Peptidyl-prolyl isomerases (PPIases) catalyze cis/trans isomerization of peptidyl-prolyl bonds, which is often rate-limiting for protein folding. SlyD is a two-domain enzyme containing both a PPIase FK506-binding protein (FKBP) domain and an insert-in-flap (IF) chaperone domain. In order to improve our understanding of the mechanism of SlyD and of FKBPs in general, we set out to analyze the kinetics, energetics, and structural basis for substrate binding and inhibition of SlyD from Thermus thermophilus (TtSlyD) using 15-residue-long unmodified peptides, which we reasoned would be better mimics of natural unfolded protein substrates than the traditionally used 4-nitroanilide tetrapeptides. In total, we obtained five structures of TtSlyDFL and three of TtSlyDΔIF at a maximum resolution of up to 1.4 Å.

Finally, we also analyzed binding of the S2, S3, and mutated variants of the S2 peptide to a chimeric TtSlyD construct, in which the IF domain is replaced by the flap loop from human FKBP12 (henceforth abbreviated TtSlyDΔIF). Interestingly, peptides derived from S2 and S3 display a dual binding mode with both a high- and a low-affinity binding site. The highest affinities were obtained for the S2 peptide with KD1 = 0.161 μM and KD2 = 2.97 μM, followed by the S3 peptide with KD1 = 0.869 μM and KD2 = 22.94 μM. A comparison of the thermodynamic fingerprints of the S2 and S3 peptides revealed that the slightly lower affinity of the S3 peptide to the IF domain is caused by a reduction in binding enthalpy (which is partly compensated by entropy), while the weaker binding of the S3 peptide to the FKBP domain is due to entropic effects. The TtSlyDFL:T1 and TtSlyDΔIF:S3 structures both show alternative binding modes. The S3 peptide binds to TtSlyDΔIF by inserting a valine instead of a proline residue into the binding pocket, which supports the conclusion that in vitro binding to the FKBP domain does not strictly require the presence of proline residues. The peptide inserts a cis-proline residue into the hydrophobic binding pocket in all cases, except in the TtSlyDΔIF:S3 structure, where a trans-valine residue is inserted instead, thus further supporting the conclusion that proline residues are not essential for binding to the FKBP domain. The non-canonical binding modes agree well with the weaker affinities of these peptides, but it is unclear if they mimic any physiologically relevant interactions. As discussed further below, this variability is intimately connected with interactions between the side chain of Y63 and the peptides bound to the FKBP domain. The FKBP12 flap loop inserted into TtSlyDΔIF in place of the IF domain adopts essentially the same conformation as in full-length FKBP12 in the case of TtSlyDΔIF:FK506, while it is partially disordered in TtSlyDΔIF:S2-W23A and TtSlyDΔIF:S3.

> MKVGQDKVVTIRYTLQVEGEVLDQGELSYLHGHRNLIPGLEEALEGREEGEAFQAHVPAEKAYGATGHPGIIPPHATLDFQVEVVKVREATPEELLHGHAHPSGHHHHHH;> RLGIVKPWNSTWFANX> MEANGLGPQGFPELKNDTFLRAAWGEETDYTPVWCMRQAGRYLPEFRETRAAQDFFSTCRSPEACCELTLQPLRRFPLDAAIIFSNILVVPQALGMEVTMVPGKGPSFPEPLREEQDLERLRDPEVVASELGYVFQAITLTRQRLAGRVPLIGFAGAPWTLMTYMVEG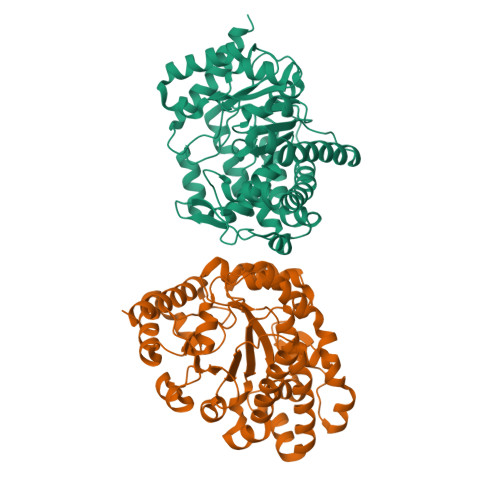GGSSTMAQAKRWLYQRPQASHQLLRILTDALVPYLVGQVVAGAQALQLFESHAGHLGPQLFNKFALPYIRDVAKQVKARLREAGLAPVPMIIFAKDGHFALEELAQAGYEVVGLDWTVAPKKARECVGKTVTLQGNLDPCALYASEEEIGQLVKQMLDDFGPHRYIANLGHGLYPDMDPEHVGAFVDAVHKHSRLLRQN> AAAAAAAAA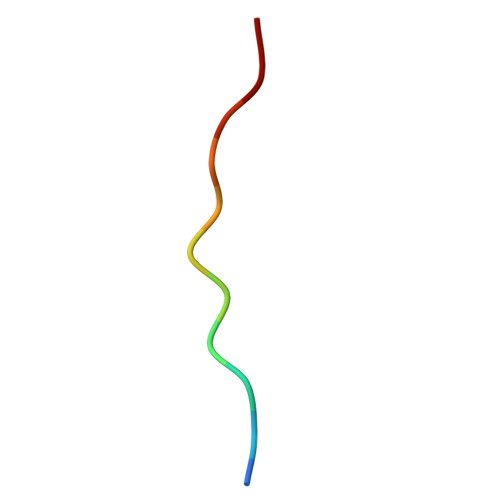AA> MSAEVIGQVEEALDTDEKEMLLFLCRDVAIDVVPPNVRDLLDILRERGKLSVGDLAELLYRVRRFDLLKRILKMDRKAVETHLLRNPHLVSDYRVLMAEIGEDLDKSDVSSLIFLMKDYMGRGKISKE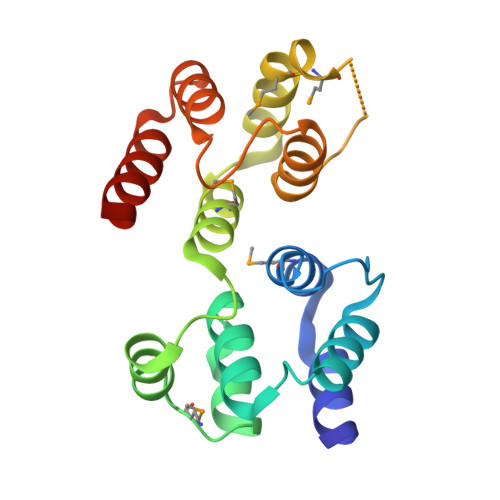KSFLDLVVELEKLNLVAPDQLDLLEKCLKNIHRIDLKTKIQKYKQSVQGAGTS> AAPAYGQPSAAMGQNMRPMNQLYPIDLLTELPPPITDLTLPPPPLVIPPERMLVPSELSNASPDYIRSTLNAVPKNSSLLKKSKLPFGLVIRPYQHLYDDIDPPPLNEDGLIVRCRRCRSYMNPFVTFIEQGRRWRCNFCRLANDVPMQMDQSDPNDPKSRYDRNEIKCAVMEYMAPKEYTLRQPPPATYCFLIDVSQSSIKSGLLATTINTLLQNLDSIPNHDERTRISILCVDNAIHYFKIPLDSENNEESADQINMMDIADLEEPFLPRPNSMVVSLKACRQNIETLLTKIPQIFQSNLITNFALGPALKSAYHLIGGVGGKIIVVSGTLPNLGIGKLQRRNESGVVNTSKETAQLLSCQDSFYKNFTIDCSKVQITVDLFLASEDYMDVASLSNLSRFTAGQTHFYPGFSGKNPNDIVKFSTEFAKHISMDFCMETVMRARGSTGLRMSRFYGHFFNRSSDLCAFSTMPRDQSYLFEVNVDESIMADYCYVQVAVLLSLNNSQRRIRIITLAMPTTESLAEVYASADQLAIASFYNSKAVEKALNSSLDDARVLINKSVQDILATYKKEIVVSNTAGGAPLRLCANLRMFPLLMHSLTKHMAFRSGIVPSDHRASALNNLESLPLKYLIKNIYPDVYSLHDMADEAGLPVQTEDGEATGTIVLPQPINATSSLFERYGLYLIDNGNELFLWMGGDAVPALVFDVFGTQDIFDIPIGKQEIPVVENSEFNQRVRNIINQLRNHDDVITYQSLY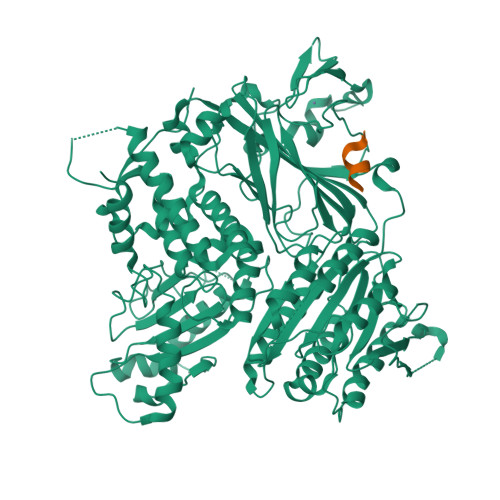IVRGASLSEPVNHASAREVATLRLWASSTLVEDKILNNESYREFLQIMKARISK;> LASLESQS> APEPGSTCRLREYYDQTAQMCCSKCSPGQHAKVFCTKTSDTVCDSCEDSTYTQLWNWVPECLSCGSRCSSDQVETQACTREQNR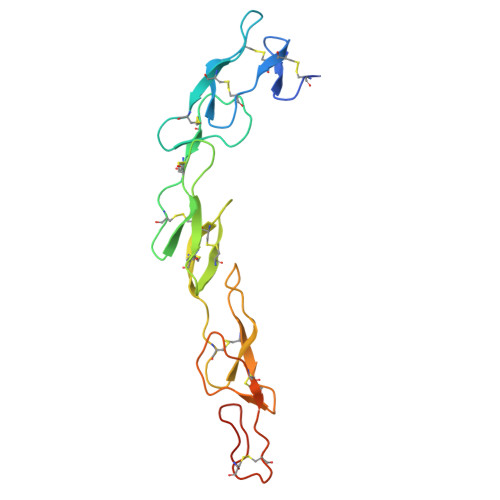ICTCRPGWYCALSKQEGCRLCAPLRKCRPGFGVARPGTETSDVVCKPCAPGTFSNTTSSTDICRPHQICNVVAIPGNASMDAVCTSTSP> MEDNYAADVQRQFNRTAFDSLYKICYNSLVQKNGSTI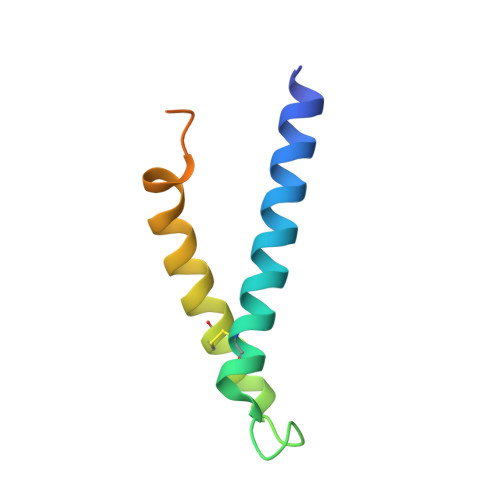DFQKQIDCHQRLIQVFAKIAPIVVKVEQDAASSGGAAAGGEDEE> MSENLKDEILEKYIPKTKKTRSGHIVIKTEETPNPEIVANTRTVPGIITARGCAYAGCKGVVMGPIKDMVHITHGPIGCSFYTWGGRRFKSKPENGTGLNFNEYVFSTDMQESDIVFGGVNKLKDAIHEAYEMFHPAAIGVYATCPVGLIGDDILAVAATASKEIGIPVHAFSCEGYKGVSQSAGHHIANNTVMTDIIGKGNKEQKKYSINVLGEYNIGGDAWEMDRVLEKIGYHVNATLTGDATYEKVQN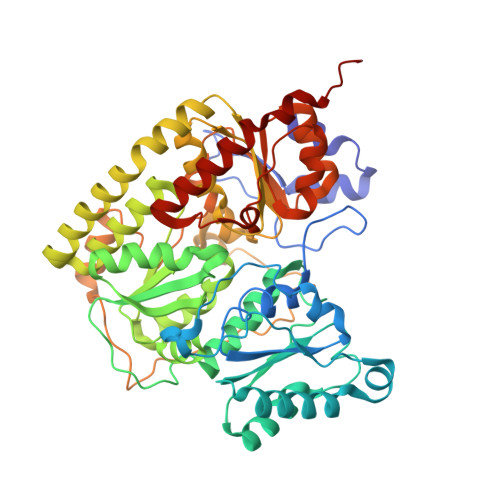ADKADLNLVQCHRSINYIAEMMETKYGIPWIKCNFIGVDGIVETLRDMAKCFDDPELTKRTEEVIAEEIAAIQDDLDYFKEKLQGKTACLYVGGSRSHTYMNMLKSFGVDSLVAGFEFAHRDDYEGREVIPTIKIDADSKNIPEITVTPDEQKYRVVIPEDKVEELKKAGVPLSSYGGMMKEMHDGTILIDDMNHHDMEVVLEKLKPDMFFAGIKEKFVIQKGGVLSKQLHSYDYNGPYAGFRGVVNFGHELVNGIYTPAWKMITPPWK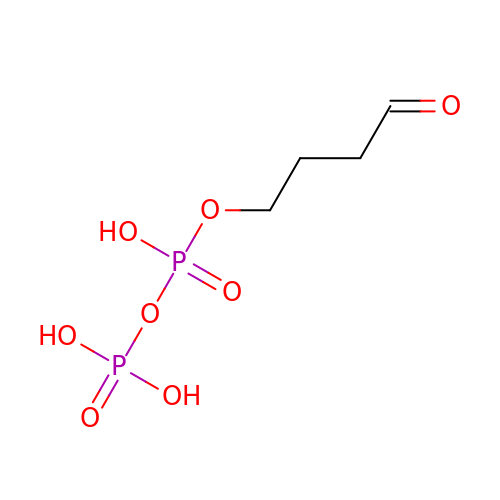4-oxobutyl trihydrogen diphosphate | C4 H10 O8 P2 | NNKWBPRTAQVCDC-UHFFFAOYSA-N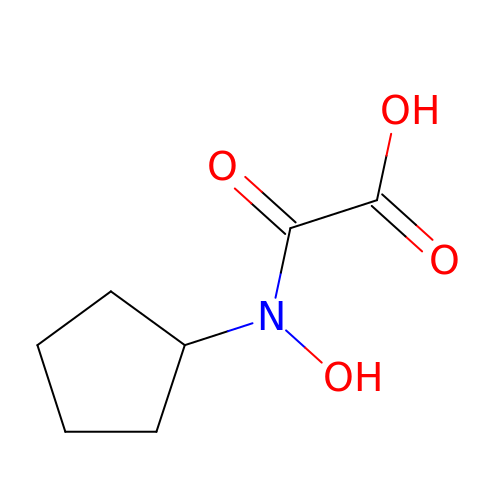[cyclopentyl(hydroxy)amino](oxo)acetic acid | C7 H11 N O4 | LBAXJZMLDPZSOL-UHFFFAOYSA-N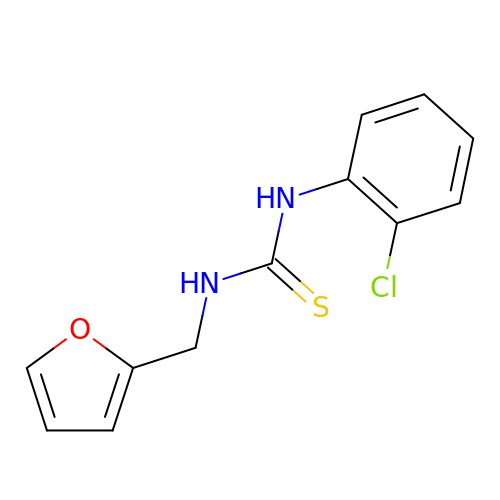N-(2-chlorophenyl)-N'-[(furan-2-yl)methyl]thiourea | C12 H11 Cl N2 O S | QDQNQQPXAIJIJW-UHFFFAOYSA-N>[2x]MLNQFPGQYSNNIFCFPPIESETKSGKKASWIICVQVVQHNTIIPITDEMFSTDVKDAVAEIFTKFFVEEGAVRISKMTRVTEGKNLGKKNATTVVHQAFKDALSKYNRHARQKRGAHTNRGMIPPMLVKYFNIIPKTFFEEETDPIVQRKRNGVRAVACQQGDGCILLYSRTEKEFLGLDNIKKELKQLYLFIDVRVYLDGELYLHRKPLQWIAGQANAKTDSSELHFYVFDCFWSDQLQMPSNKRQQLLTNIFKQKEDLTFIHQVENFSVKNVDEALRLKAQFIKEGYEGAIVRNANGPYEPGYNNYHSAHLAKLKPLLDAEFILVDYTQGKKGKDLGAILWVCELPNKKRFVVTPKHLTYADRYALFQKLTPALFKKHLYGKELTVEYAELSPKTGIPLQARAVGFREPINVLEII

AsfvLIG catalyzes the DNA ligation reaction during the base excision repair (BER) process of ASFV genome. AsfvLIG is composed of 419 amino acids and is one of the smallest DNA ligases identified to date. However, unlike the homologous proteins (such as HsLIG1 and SusLIG1), the fidelity of AsfvLIG is very low. By solving four AsfvLIG:DNA complex structures, including the non-catalytic open form and the catalytic closed forms, we showed that the NTD, AD, and OB domains of AsfvLIG undergo a large conformational change during the catalytic assembly.

Crystals of the non-catalytic form structure were grown in the presence of ATP but without Mg2+, which is an essential cofactor of the adenylation reaction. We found that the non-catalytic structure adopts an extended fold and the ATP is bound by the AD domain and stabilized by various interactions. Besides hydrophobic stacking with the side chains of Ile294 and Phe232, the nucleobase of ATP forms one hydrogen bond (H-bond) with Gln149, via the N6 and OE1 atoms. The sugar pucker 2′-OH group and the oxygen atoms of the phosphate groups form H-bonds with the side chains of Lys151, Glu203, and Lys316. In the non-catalytic form structure, the substrate DNA was bound by the NTD domains of two AsfvLIG molecules and adopts regular B-form conformation; though the DNA adopts a regular B-form conformation at the two ends, it was significantly bent and unwound around the nick site in the catalytic form complex. The ATP was captured in the active site of the non-catalytic form AsfvLIG:DNA structure. The catalytic Lys residue (Lys151) and ATP-interacting residues of AsfvLIG are highly conserved in the homologous proteins. A bound ATP molecule is present in the non-catalytic structure, demonstrating that AsfvLIG has ATP binding and catalytic mechanism commonly shared by many other ligases.> ITGRPEWIWLALGTALMGLGTLYFLVKGMGVSDPDAKKFYAITTLVPAIAFTMYLSMLLGYGLTMVPFGGEQNPIYWARYADWLFTTPLLLLDLALLVDADQGTILALVGADGIMIGTGLVGALTKVYSYRFVWWAISTAAMLYILYVLFFGFTSKAESMRPEVASTFKVLRNVTVVLWSAYPVVWLIGSEGAGIVPLNIETLLFMVLDVSAKVGFGLILLRSRAIFGEAE

The best characterized system is bacteriorhodopsin (bR), a light-driven proton pump, due to its biochemical robustness. The retinal chromophore of bR (Halobacterium salinarum) is linked to the side chain of Lys216 via a protonated Schiff base (PSB). Photon absorption by all-trans retinal triggers a functional photocycle consisting of a series of distinct spectroscopic intermediates (I→J→K→L→M→N→O) with sub-ps (I), ps (J), µs (K, L) and ms (M, N, O) lifetimes. Deprotonation of the Schiff base of photoisomerized 13-cis retinal and protonation of Asp85 during the L→M transition ultimately results in proton translocation to the extracellular side of the membrane.

For comparison, we also collected data of the dark state. In the dark state, the polyene chain of all-trans retinal is largely planar (C6-C13) with a slightly pre-twisted C13=C14 double bond when no planarity for the atoms around this bond is enforced during refinement (torsion angle −150°, “dark-unrestrained” structure), in line with computational work (−160°). In the dark state, PSB forms a hydrogen bond with Wat402 (2.8 Å).>MPREYEFAEKILFTEEEIRTRIKEVAKRIADDYKGKGLRPYVNPLVLISVLKGSFMFTADLCRALCDFNVPVRMEFICVSSYGEGLTSSGQVRMLLDTRHSIEGHHVLIVEDIVATALTLNYLYHMYFTRRPASLKTVVLLDKREGRRVPFSADYVVANIPNAFVIGYGLDYDDTYRELRDIVVLRPEVYAEREAARGKKQ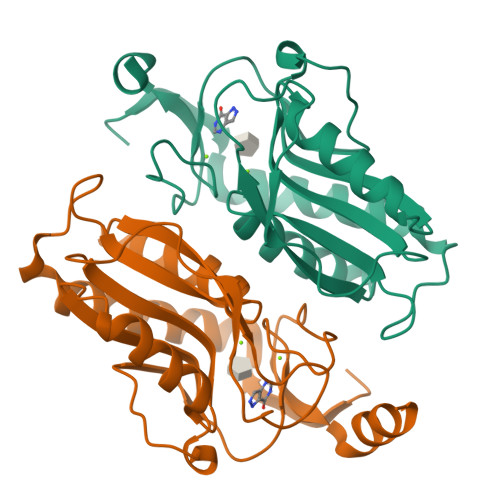RAIGSADTDRDAKREFHSKY[2x]> PISPIETVPVKLKPGMDGPKVKQWPLTEEKIKALVEICTEMEKEGKISKIGPENPYNTPVFAIKKKDSTKWRKLVDFRELNKRTQDFWEVQLGI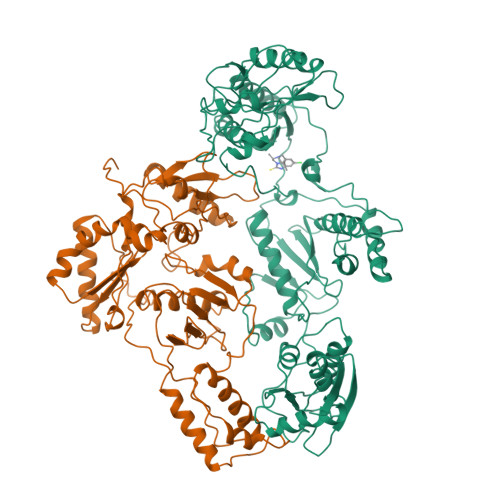PHPAGLKKKKSVTVLDVGDAYFSVPLDEDFRKYTAFTIPSINNETPGIRYQYNVLPQGWKGSPAIFQSSMTKILEPFKKQNPDIVIYQYMDDLYVGSDLEIGQHRTKIEELRQHLLRWGLTTPDKKHQKEPPFLWMGYELHPDKWTVQPIVLPEKDSWTVNDIQKLVGKLNWASQIYPGIKVRQLSKLLRGTKALTEVIPLTEEAELELAENREILKEPVHGVYYDPSKDLIAEIQKQGQGQWTYQIYQEPFKNLKTGKYARMRGAHTNDVKQLTEAVQKITTESIVIWGKTPKFKLPIQKETWETWWTEYWQATWIPEWEFVNTPPLVKLWYQLEKEPIVGAETFYVDGAANRETKLGKAGYVTNKGRQKVVPLTNTTNQKTELQAIYLALQDSGLEVNIVTDSQYALGIIQAQPDKSESELVNQIIEQLIKKEKVYLAWVPAHKGIGGNEQVDKLVSAGIRK;> PISPIETVPVKLKPGMDGPKVKQWPLTEEKIKALVEICTEMEKEGKISKIGPENPYNTPVFAIKKKDSTKWRKLVDFRELNKRTQDFWEVQLGIPHPAGLKKKKSVTVLDVGDAYFSVPLDEDFRKYTAFTIPSINNETPGIRYQYNVLPQGWKGSPAIFQSSMTKILEPFKKQNPDIVIYQYMDDLYVGSDLEIGQHRTKIEELRQHLLRWGLTTPDKKHQKEPPFLWMGYELHPDKWTVQPIVLPEKDSWTVNDIQKLVGKLNWASQIYPGIKVRQLSKLLRGTKALTEVIPLTEEAELELAENREILKEPVHGVYYDPSKDLIAEIQKQGQGQWTYQIYQEPFKNLKTGKYARMRGAHTNDVKQLTEAVQKITTESIVIWGKTPKFKLPIQKETWETWWTEYWQATWIPEWEFVNTPPLVKLWY>[2x]MGSSHHHHHHSSENLYFQGGGMVSQLAV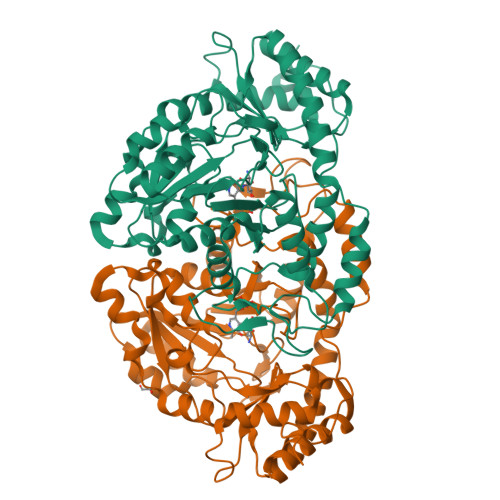KGGEALRTRPWPAWPQPAPGVPDAVADVLGSGRWSISGPYRGTESYERRFARAFAAYNGVPHCVPAASGTASLMLALEACGIGAGDEVIVPGLSWVASGSTILGVNAVPIFCDVDPDTLCLSPEAVEAAITEHTRAIVVVHLYSALADMDALSAIAERHGLPLIEDCAQAHGATYRGVKVGALATAGTFSMQHSKVLTSGEGGAVITRDEDFARRVEHLRADGRCLSAVPPAPGAMELVETGELMGNNRCLSEFQAAILAEQLTILDEQNETRRANAAHLDGLLGELGLRPQTTSDGTTSRTYYTYAVRLPDGVLEDVPVTDVSCALTAELGFPVLPSYAPIPANRLYTPHTRRRYTLGLDHERRIDPKRFALPVCEDAARRTVTLHHAALLGDADDMGDIAAAFAKVLRHGAGLMH>GKAFDDGAFTGIREINLSYNKETAIGDFQVVYDLNGSPYVGQNHKSFITGFTPVKISLDFPSEYIMEVSGYTGNVSGYVVVRSLTFKTNKKTYGPYG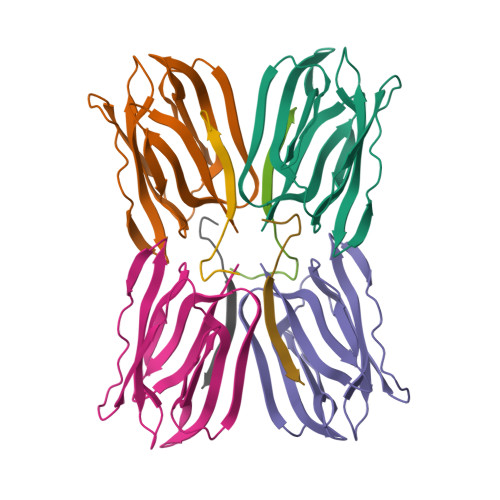VTSGTPFNLPIENGLIVGFKGSIGYWLDYFSMYLSL[4x];>NEQSGISQTVIVGPWGAK[4x]2ALPHA-METHYL-1ALPHA,25-DIHYDROXY-VITAMIN D3 | C28 H46 O3 | 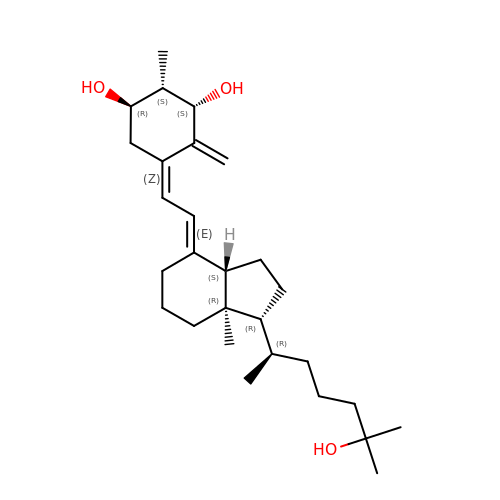PSWKLSOBPNHZSY-GEMNOXHFSA-N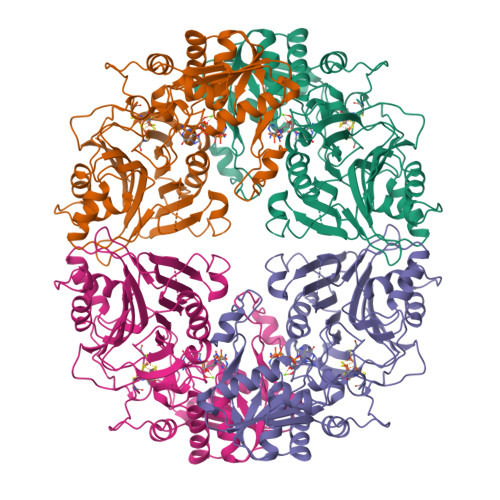>[4x]CGVFGIWGHEEAPQITYYGLHSLQHRGQEGAGIVATDGEKLTAHKGQGLITEVFQNGELSKVKGKGAIGHVRYATAGGGGYENVQPLLFRSQNNGSLALAHNGNLVNATQLKQQLENQGSIFQTSSDTEVLAHLIKRSGHFTLKDQIKNSLSMLKGAYAFLIMTETEMIVALDPNGLRPLSIGMMGDAYVVASETCAFDVVGATYLREVEPGEMLIINDEGMKSERFSMNINRSICSMEYIYFSRPDSNIDGINVHSARKNLGKMLAQESAVEADVVTGVPDSSISAAIGYAEATGIPYELGLIKNRYVGRTFIQPSQALREQGVRMKLSAVRGVVEGKRVVMVDDSIVRGTTSRRIVTMLREAGATEVHVKISSPPIAHPCFYGIDTSTHEELIASSHSVEEIRQEIGADTLSFLSVEGLLKGIGRKYDDSNCGQCLACFTGKYPTEIYQDTVLPHVK>ANFIEKITYLGTPAIKAGNEHLEMIVVPEWGSNVISLVDKTTNV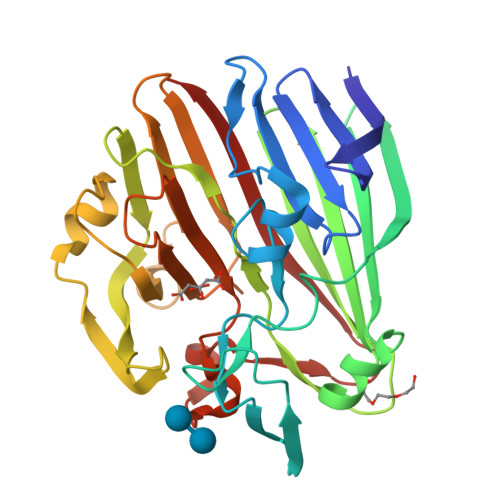QLLREPETAESFHDTPTLYGIPILFPPNRISDGTFSFRGRTYHFDINEKDKHNHLHGFLYHEKWNVVTTKQTDEGVIVETEIDLSELPHVQKQFPHHAVVRMTYTIKENTLFKHATVMNKGKEAFPWGIGYHTTFIFPAESSLFSLTADQQWELDERLLPTGKLMDVPYKEALHEGMDLRHKQLDDVFLSSYQKRGGENQAVIYHQHAHISIIYKADEQFKHWVVYNADGKQGYLCPEPYTWVTNAVNLDLPSSLTGLQVLEPGEETTAKSSITIELNHQ[2x]>MSVLPFLRIYAPLNAVLAAPGLLAVAALTIPDMSGRSRLALAALLAVIWGAY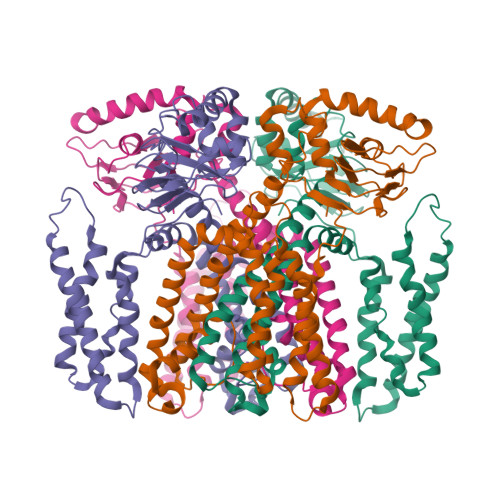LLQLAATLLKRRAGVVRDRTPKIAIDVLAVLVPLAAFLLDGSPDWSLYCAVWLLKPLRDSTFFPVLGRVLANEARNLIGVTTLFGVVLFAVALAAYVIERDIQPEKFGSIPQAMWWAVVTLSTTGYGDTIPQSFAGRVLAGAVMMSGIGIFGLWAGILATGFYQEVRRGDFVRNWQLVAAVPLFQKLGPAVLVEIVRALRARTVPAGAVICRIGEPGDRMFFVVEGSVSVATPNPVELGPGAFFGEMALISGEPRSATVSAATTVSLLSLHSADFQMLCSSSPEIAEIFRKTALERRGAAASA[4x]> QFAKPEDAVKYR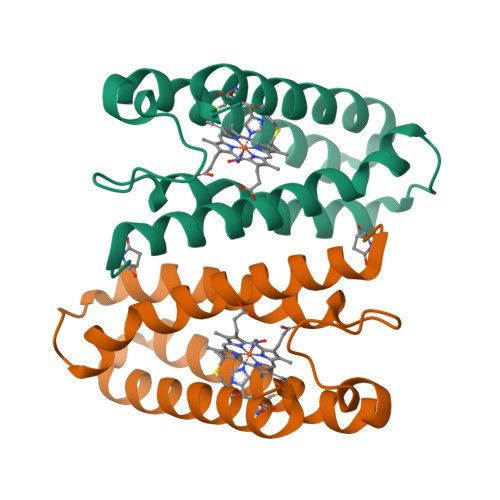QSAITLMASHFGRMTPVVKGQAPYDAAQIKANVEVLKTLSALPWAAFGPGTEGGDARPEIWSDAASFKQKQQAFQDNIVKLSAAADAGDLDKLRAAFGDVGASCKACHDAYRKK> GHMTGVESFMTKQDTTGKIISIDTSSL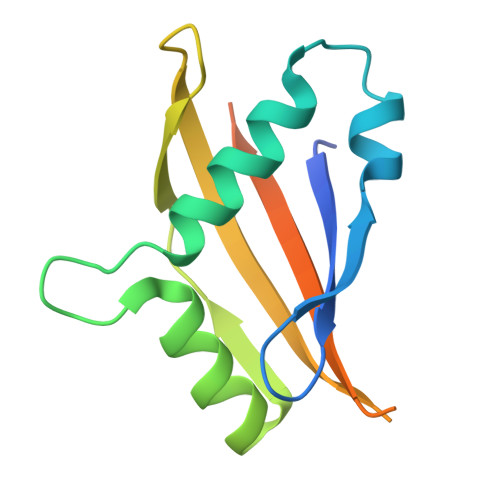RAAGRTGWEDLVRKCIYAFFQPQGREPSYARQLFQEVMTRGTASSPSYRFILNDGTMLSAHTRCKLCYPQSPDMQPFIMGIHIIDREHSGLSPQDDTNSGMSIPR>[4x]FQVPMSNLLTVHQNLPALPVDATSDEVRKNLMDMFRDRQAFSEHTWKMLLSVCRSWAAWCKLNNRKWFPAEPEDVRDYLLYLQARGLAVKTIQQHLGQLNMLHRRSGLPRPSDSNAVSLVMRRIRKENVDAGERAKQALAFERTDFDQVRSLMENSDRCQDIRNLAFLGIAYNTLLRIAE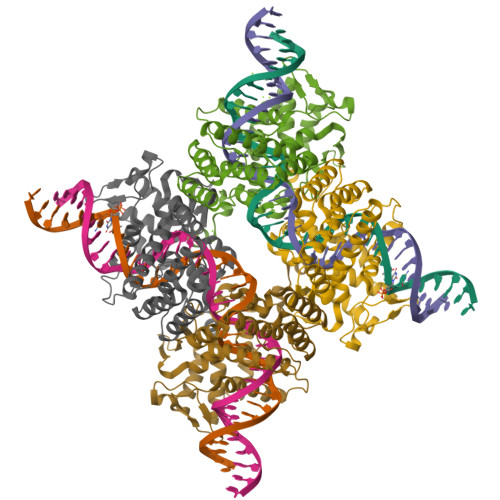IARIRVKDISRTDGGRMLIHIGRTKTLVSTAGVEKALSLGVTKLVERWISVSGVADDPNNYLFCRVRKNGVAAPSATSQLSTRALEGIFEATHRLIYGAKDDSGQRYLAWSGHSARVGAARDMARAGVSIPEIMQAGGWTNVNIVMNYIRNLDSETGAMVRLLEDGD>[2x]GVSGSKGQKLFVSVLQRLLSERGLHVKESSAIEFYQFLIKVSPWFPEEGGLNLQDWKRVGREMKRYAAEHGTDSIPKQAYPIWLQLREILT

Mouse mammary tumor virus (MMTV), a causative agent of mammary breast cancer and T cell lymphomas in mice, is a representative of the Betaretrovirus genus. The N-terminal domain of Gag, matrix (MA) protein, is responsible for Gag targeting and PM binding. Myristoylation of MA and the highly basic patch of amino acids located near its N-terminus mediate the interaction of Gag with the PM. Here, we investigated the role of myristoylation on oligomerization of MMTV MA and determined the crystal structure of myr(+) MMTV MA, which represents the first X-ray structure of a myr(+) retroviral MA protein.

The protein crystallized in the P3121 space group with two molecules in the asymmetric unit. The final dataset was collected to 1.57 Å resolution, and the final model was refined to R = 22.6 % (Rfree = 26.3 %). In the refined structure, myristoyl groups and their connections to the N-terminal glycines were well-defined in the electron density map, as were the first 91 of 111 amino acid residues. The monomeric subunit is a helical bundle comprising five alpha helices and a single-turn 310-helix (helix 5). The CTRS region (spanning residues 45–62) is accessible on the surface of the molecule in an orientation similar to that observed for M-PMV MA. Interestingly, the myristoyl group of one of the dimer-forming MA molecules is not buried in the hydrophobic core of the protein chain to which it is covalently attached, as is common for the sequestered form of myr(+) MA proteins. Instead, the myristoyl group is sequestered in the hydrophobic pocket formed by the interface of both MA molecules in the asymmetric dimer unit. This interface is formed predominantly by helices 1 and 3. However, the myristoyl group of the second MA molecule in the dimer extrudes into the neighboring dimer unit. Therefore, the two nearest dimer units in the crystal are interconnected by two myristoyl groups, forming a tetramer of MA molecules around the two-fold axis of the P3121 space group.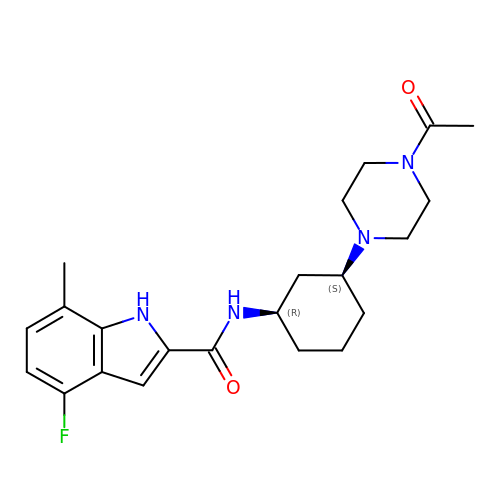N-[(1R,3S)-3-(4-acetylpiperazin-1-yl)cyclohexyl]-4-fluoro-7-methyl-1H-indole-2-carboxamide | C22 H29 F N4 O2 | PGNLXEBQMQHFNK-SJORKVTESA-N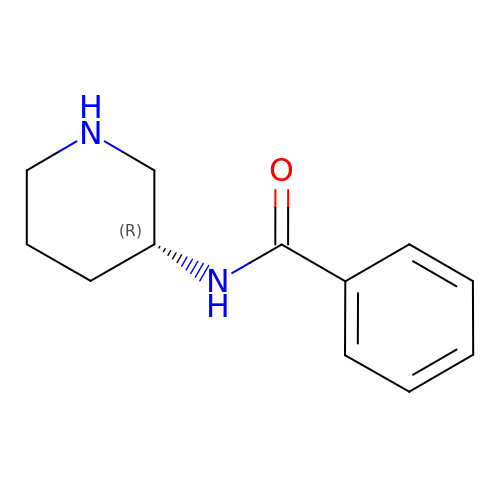N-[(3R)-piperidin-3-yl]benzamide | C12 H16 N2 O | ZFLKDMGBVZHBAC-LLVKDONJSA-N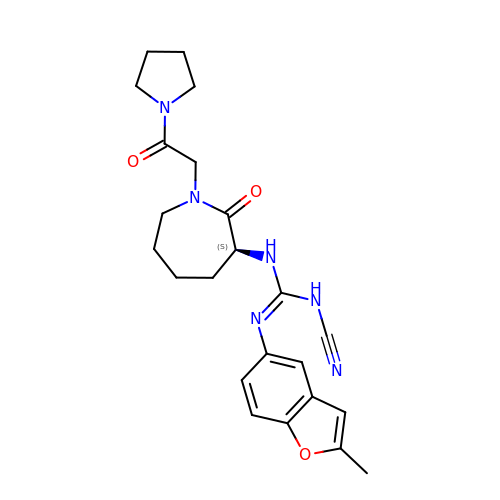1-cyano-2-(2-methyl-1-benzofuran-5-yl)-3-[(3S)-2-oxo-1-(2-oxo-2-pyrrolidin-1-ylethyl)azepan-3-yl]guanidine | C23 H28 N6 O3 | BQUXAJWDRCSKFN-IBGZPJMESA-N>[4x]HHHHHHMSAIKPDMKINLRMEGNVNGHHFVIDGDGTGKPFEGKQSMDLEVKEGGPLPFAFDILTT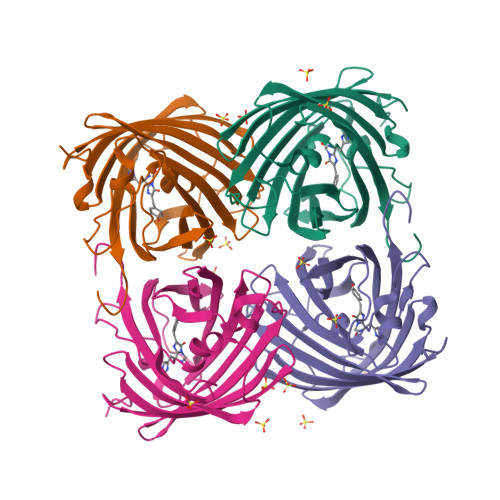AFHYGNRVFAEYPDHIQDYFKQSFPKGYSWERSLTFEDGGICIARNDITMEGDTFYNKVRFHGVNFPANGPVMQKKTLKWEPSTEKMYVRDGVLTGDITMALLLEGNAHYRCDSRTTYKAKEKGVKLPGYHLVDHCIEILSHDKDYNKVKLYEHAVAHSGLPDNARR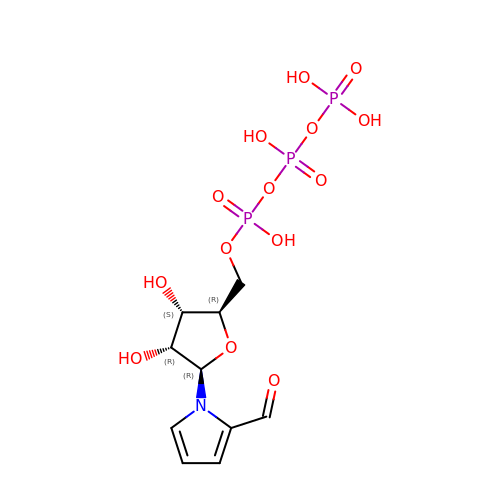1-{5-O-[(S)-hydroxy{[(R)-hydroxy(phosphonooxy)phosphoryl]oxy}phosphoryl]-beta-D-ribofuranosyl}-1H-pyrrole-2-carbaldehyde | C10 H16 N O14 P3 | CLXMUGOYLDUWBK-PBVVMKELSA-N> ATYAMGSMRVLLALHDRAPQLKISDDRLTVVGEKGYSMVRASHGVRKGAWYFEITVDEMPPDTAARLGWSQPLGNLQAPLGYDKFSYSWRSKKGTKFHQSIGKHYSSGYGQGDVLGFYINLPEDTISGRGSEIIFYKNGVNQGVAYKDIFEGVYFPAISLYKSCTVSINFGPCFKYPPKDLTYRPMSDMGWGAVVEHTLADVLYHVETEVDGRR;>GMEPEQMLEGQTQVAENPHSEYGLTDNVERIVENEKINAEKSSKQKVDLQSLPTRAYLDQTVVPILLQGLAVL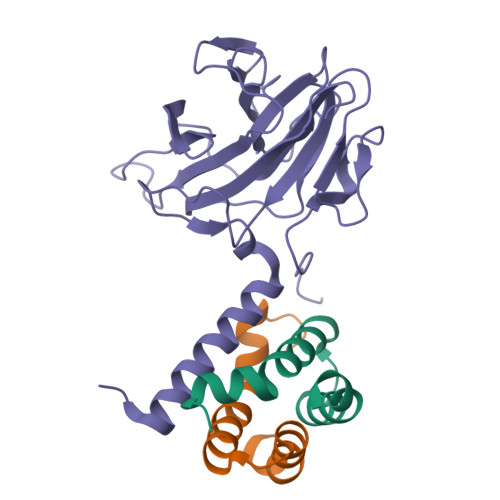AKERPPNPIEFLASYLLKNKAQFEDRN[2x]> AGLVPRGSHMKILVIQGPNLNMLGHRDPRLYGMVTLDQIHEIMQTFVKQGNLD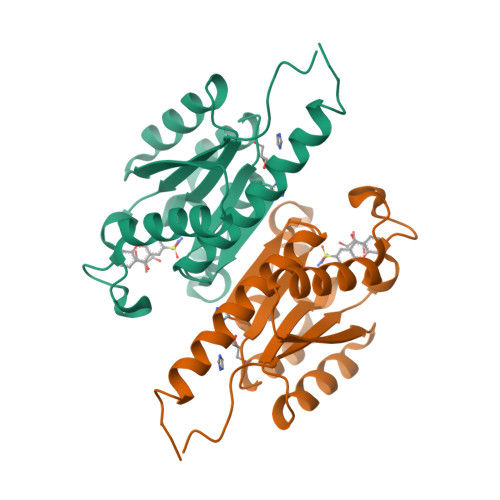VELEFFQTNFEGEIIDKIQESVGSEYEGIIINPGAFSHTSIAIADAIMLAGKPVIEVHLTNIQAREEFRKNSYTGAACGGVIMGFGPLGYNMALMAMVNILAEMKAFQEAQKNNPNNPINNQK>MAKKNKMKPRELREAQKKARQLKAAEINNNAAPAIAAMPAAEVIAPVAEKKKSSVKAAGMKSILVSENKMYITSFGKGNSAVLEYEVDNNDYNKTQLSSKDNSNIELGDVNEVNITFSSKHGFGSGVEINTSNPTHRSGESSPVRGDMLGLKSELEKRFFGKTFDDNIHIQLIYNILDIEKILAVYVTNIVYALNNMLGIKDSESYDDFMGYLSARNTYEVFTHPDKSNLSDKVKGNIKKSLSKFNDLLKTKRLGYFGLEEPKTKDTRASEAYKKRVYHMLAIVGQIAQCVFHDKSGAKRFDLYSFINNIDPEYRDTLDYLVEERLKSINKDFIEGNKVNISLLIDMMKGYEADDIIRLYYDFIVLKSQKNLGFSIKKLREKMLEEYGFRFKDKQYDSVRSKMYKLMDFLLFCNYYRNDVAAGEALVRKLRFSMTDDEKEGIYADEAAKLWGKFRNDFENIADHMNGDVIKELGKADMDFDEKILDSEKKNASDLLYFSKMIYMLTYFLDGKEINDLLTTLISKFDNIKEFLKIMKSSAVDVECELTAGYKLFNDSQRITNELFIVKNIASMRKPAASAKLTMFRDALTILGIDDNITDDRISEILKLKEKGKGIHGLRNFITNNVIESSRFVYLIKYANAQKIREVAKNEKVVMFVLGGIPDTQIERYYKSCVEFPDMNSSLEAKRSELARMIKNISFDDFKNVKQQAKGRENVAKERAKAVIGLYLTVMYLLVKNLVNVNARYVIAIHCLERDFGLYKEIIPELASKNLKNDYRILSQTLCELCDDRNESSNLFLKKNKRLRKCVEVDINNADSSMTRKYANCIAHLTVVRELKEYIGDIRTVDSYFSIYHYVMQRCITKRGDDTKQEEKIKYEDDLLKNHGYTKDFVKALNSPFGYNIPRFKNLSIEQLFDRNEYLTEKLEHHHHHH[2x]

Cas13d is a class 2 type VI-D CRISPR-Cas RNA-guided RNase. Cas13 family is the only family of class 2 Cas enzymes known to exclusively target single-stranded RNA. Analogously to the other members of the Cas13 superfamily, Cas13d also contains two R-X4-H HEPN motifs, but bears little overall similarity to the amino acid sequences of Cas13a and Cas13b. Owing to its biochemical properties, especially small size, lack of constraints on the target flanking sequences, and highly efficient and specific target RNA cleavage, Cas13d is a promising candidate for RNA engineering and editing.

In order to understand the structural basis of pre-crRNA processing and mature crRNA recognition by Cas13d, we solved the crystal structure of the uncultured Ruminococcus sp. Cas13d (UrCas13d, also known as RspCas13d)-crRNA complex at 2.15 Å resolution using the single-wavelength anomalous diffraction method. The binary complex was obtained by the selenomethionine (SeMet)-derived UrCas13d (R288A/R823A) mutant co-expressed with CRISPR RNA in vivo. The SeMet-labeled structure was subsequently used as a model to solve the crystal structure of the unlabeled UrCas13d (R288A/R823A) binary complex at 1.86 Å resolution using the molecular replacement method. In line with the previous studies, the mature crRNA containing a 30-nt repeat region was determined in the high-resolution UrCas13d binary complexes. Although the conventional bilobed architecture consisting of a recognition (REC) lobe and a nuclease (NUC) lobe is still discernible in UrCas13d, its compact structure blurs this bilobed notion to certain extent. The REC lobe consists of the N-terminal domain (NTD) and Helical-1 domain. The NUC lobe consists of two HEPN domains (HEPN-1 and HEPN-2) and Helical-2 domain. The mature crRNA is sandwiched within a positively charged channel formed by the REC and NUC lobes.>MSQPRTPEQALDTPGDCPPGRRDEDAGEGIQCSQRMLSFSDALLSIIATVMILPVTHTEISPEQQFDRSVQRLLATRIAVYLMTFLIVTVAWAAHTRLFQVVGKTDDTLALLNLACMMTITFLPYTFSLMVTFPDVPLGIFLFCVCVIAIGVVQALIVGYAFHFPHLLSPQIQRSAHRALYRRHVLGIVLQGPALCFAAAIFSLFFVPLSYLLMVTVILLPYVSKVTGWCRDRLLGHREPSAHPVEVFSFDLHEPLSKERVEAFSDGVYAIVATLLILDICEDNVPDPKDVKERFSGSLVAALSATGPRFLAYFGSFATVGLLWFAHHSLFLHVRKATRAMGLLNTLSLAFVGGLPLAYQQTSAFARQPRDELERVRVSCTIIFLASIFQLAMWTTALLHQAETLQPSVWFGGREHVLMFAKLALYPCASLLAFASTCLLSRFSVGIFHLMQIAVPCAFLLLRLLVGLALATLRVLRGLARPEHPPPAPTGQDDPQSQLLPAPC[2x]

Transmembrane protein 175 (TMEM175) was recently identified as a constitutively-active potassium (K+) selective channel expressed in lysosomal membranes responsible for establishing a membrane potential across the lysosomal membrane. TMEM175 is implicated in cellular proteostasis and its mutation is associated with the development of Parkinson’s disease through a yet unknown mechanism, underscoring the importance of this channel to regulation of cellular homeostasis. TMEM175 is evolutionarily distinct from known K+ channels, displaying a unique membrane topology as well as lacking the conserved TVGYG selectivity filter present in canonical K+ channels such as shaker K+, BK and KcsA. Consequently, the density map revealed that while hTMEM175 is homodimeric, similarities between the two 6-helix repeat domains result in a pseudo-four-fold symmetric architecture.

To investigate the mechanisms that govern hTMEM175 function, we collected cryo-EM images of hTMEM175 purified in 150 mM K+. Three-dimensional classification revealed that two conformations were present among the imaged particles; class 1, which was resolved at a resolution of 2.6 Å, and class 2, which was resolved at a resolution of 3.0 Å. To better understand the functional states of the two conformations resolved in our data sets, we next superimposed the class 1 and class 2 structures determined in the presence of K+. Overall, the two classes are very similar, with an all-atom RMSD of 0.9 Å. In contrast to the rigid cytoplasmic side, differences between the two classes can be readily detected on the luminal side of the channel. When viewed from the luminal side of the channel, the ends of the transmembrane helices in the class 2 structure are rotated in a clockwise manner compared to their positions in class 1. The luminal loops between the transmembrane helices also adopt different conformations, with the loop between TM9 and TM10 undergoing the largest change. In class 2, the last turn of TM9 is unwound and moves nearly 12 Å from its position adjacent to the loop between TM11 and TM12 in class 1 to interact with the loop between TM1 and TM2. The comparison revealed four overlapping peaks in the class 1 maps and three in the class 2 maps. Identification of the ion-binding sites enabled us to tentatively assign the two conformations as an open state and a closed state.> MKIVYWSGTG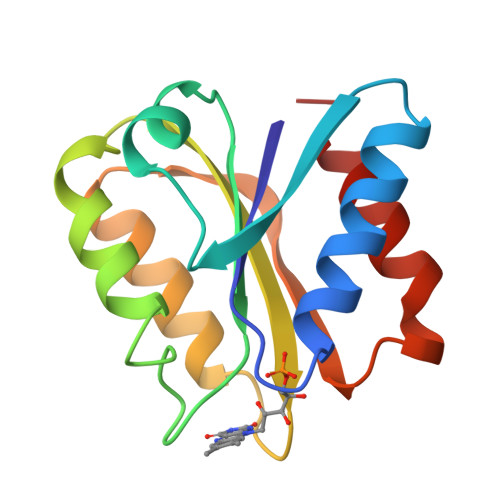NTEKMAELIAKGIIESGKDVNTINVSDVNIDELLNEDILILGCSAMADEVLEESEFEPFIEEISTKISGKKVALFGSYGWGDGKWMRDFEERMNGYGCVVVETPLIVQNEPDEAEQDCIEFGKKIANI4-(2-AMINO-5-{4-[(DIMETHYLAMINO)METHYL]THIOPHEN-2-YL}PYRIDIN-3-YL)-2-{(1R)-1-[2-(TRIFLUOROMETHYL)PHENYL]ETHOXY}BENZAMIDE 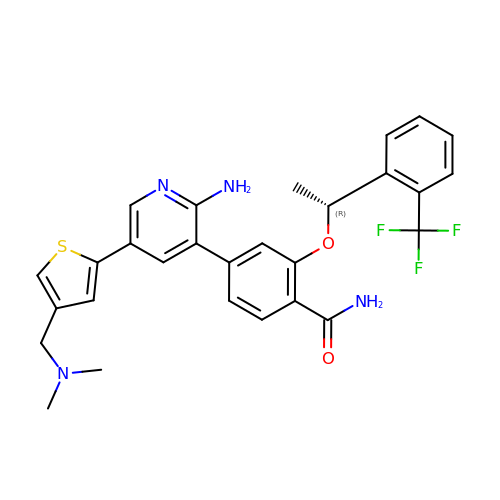| C28 H27 F3 N4 O2 S | DNZGEPPZYMAFLN-MRXNPFEDSA-N> XKPNG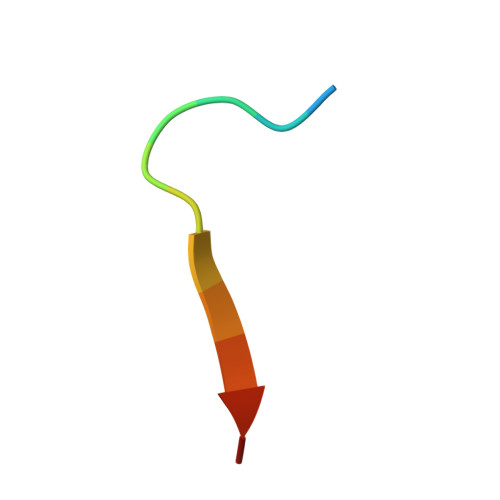LLITDFPX>[2x]GPGSMAGVDKAMVTLSNGVKMPQFGLGVWQSPAGEVTENAVKWALCAGYRHIDTAAIYKNEESVGAGL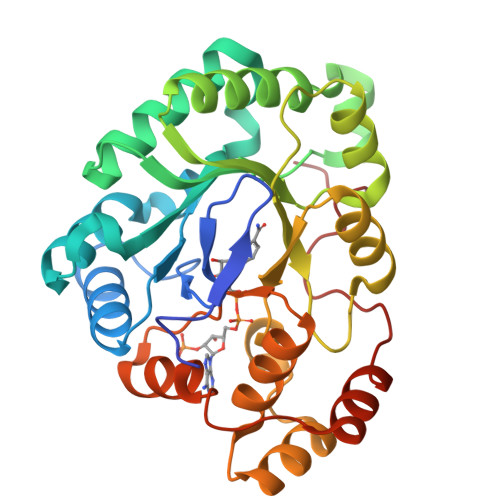RASGVPREDVFITTKLWNTEQGYESTLAAFEESRQKLGVDYIDLYLIHWPRGKDILSKEGKKYLDSWRAFEQLYKEKKVRAIGVSNFHIHHLEDVLAMCTVTPMVNQVELHPLNNQADLRAFCDAKQIKVEAWSPLGQGKLLSNPILSAIGAKYNKTAAQVILRWNIQKNLITIPKSVHRERIEENADIFDFELGAEDVMSIDALNTNSRYGPDPDEAQF> MVFESELLLQRRLATTALKQPKELGYYSTNVGGELKVMD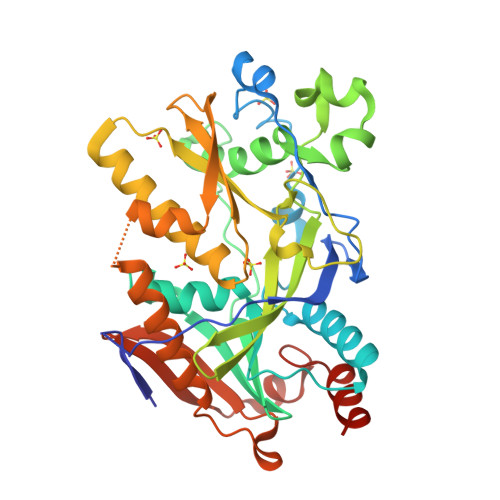ESNLSYYYLPDADIEKHIDLSAGARKFQDEQAEAEDDTGSLHGLLQTLMEYERRKSKKVNADIIAFRGQVKRLIHCAFGGHATDVDMYVMSFDGQLFIRAARKKLEFPTSPRESWAYLAYYSGYKFERMALLDRPVAETPREVLESRGKQVVRNGPQYKTVVRTGVGEHKLVLGAEVDGIFDFREPTGDNLKHYVELKVAKKVQTLKDATNFEQKLFSVWLQCFLVGINRVIIGFRDEKFVLKSVEEFSTSEIPLLLKSTGLRNACVDAIKWYGALTKWLCELPRGPEDDFKLYRLSCSRGALHLRQLHDEDLANGDDIIPGWFREWRRSLSKSHGS2-[(4-methoxybenzyl)amino]ethanesulfonic acid | C10 H15 N O4 S | 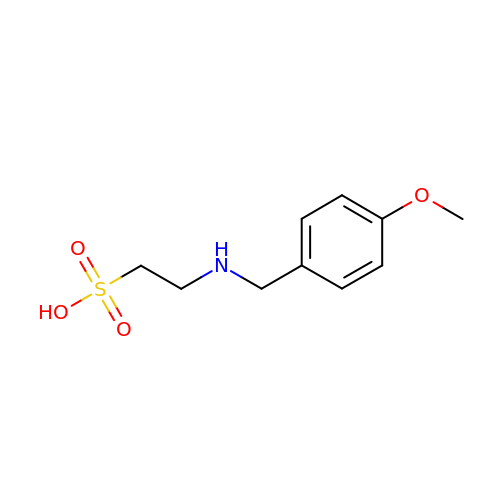AYTRHBSMOPVTHD-UHFFFAOYSA-N>GSQIPASEQETLVRPKPLLLKLLKSVGAQKDTYTMKEVLFYLGQYIMTKRLYDEKQQHIVYCSNDLLGDLFGVPSFSVKEHRKIYTMIYRNLVVVNQQESSDSGTSV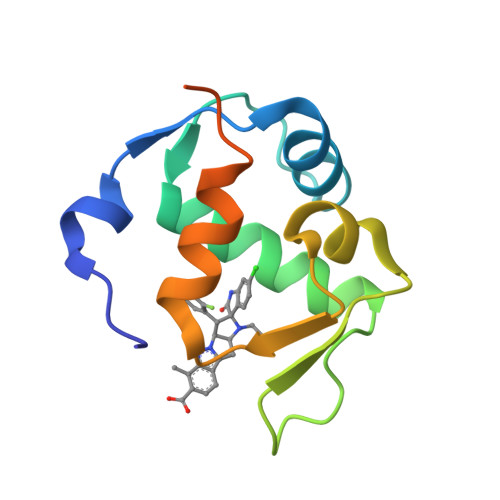SEN[3x]> MSTYEGRWKTVKVEIEDGIAFVILNRPERRNAMSPTLNREMIDVLETLEQDPAAGVLVLTGAGEAWTAGMDLKEYFREVDAGPEILQEKIRREASQWQWKLLRMYAKPTIAMVNGWCFGGGFSPLVACDLAICADEATFGLSEINWGIPPGNLVSKAMADTVGHRQSLYYIMTGKTFGGQKAAEMGLVNESVPLAQLREVTIELARNLLEKNPVVLRAAKHGFKRCRELTWEQNEDYLYAKLDQSRLLDTEGGREQGMKQFLDDKSI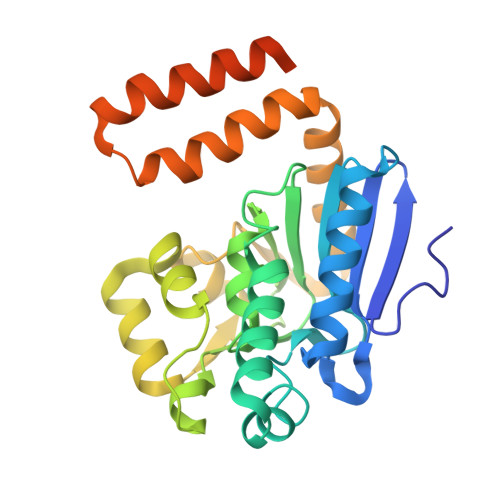KPGLQAYKR> NAINPRLTPWTYRNTSFSSLPLTGENPGAWALVRDNSAKGITAGSGSQQTTYDPTRTEAALTASTTFALRRYDLAGRALYDLDFSKLNPQTPTRDQTGQITFNPFGGFGLSGAAPQQWNEVKNKVPVEVAQDPSNPYRFAVLLVPRSVVYYEQLQRGLGLPQQRTESGQNTSTTGAMFGLKVKNAEADTAKSNEKLQGAEATGSSTTSGSGQSTQRGGSSGDTKVKALKIEVKKKSDSEDNGQLQLEKNDLANAPIKRSEESGQSVQLKADDFGTALSSSGSGGNSNPGSPTPWRPWLATEQIHKDLPKWSASILILYDAPYARNRTAIDRVDHLDPKAMTANYPPSWRTPKWNHHGLWDWKARDVLLQTTGFFNPRRHPEWFDGGQTVADNEKTGFDVDNSENTKQGFQKEADSDKSAPIALPFEAYFANIGNLTWFGQALLVFGGNGHVTKSAHTAPLSIGVFRVRYNATGTSATVTGWPYALLFSGMVNKQTDGLKDLPFNNNRWFEYVPRMAVAGAKFVGRELVLAGTITMGDTATVPRLLYDELESNLNLVAQGQGLLREDLQLFTPYGWANRPDLPIGAWSSSSSSSHNAPYYFHNNPDWQDRPIQNVVDAFIKPWEDKNGKDDAKYIYPYRYSGMWAWQVYNWSNKLTDQPLSADFVNENAYQPNSLFAAILNPELLAALPDKVKYGKENEFAANEYERFNQKLTVAPTQGTNWSHFSPTLSRFSTGFNLVGSVLDQVLDYVPWIGNGYRYGNNHRGVDDITAPQTSAGSSSGISTNTSGSRSFLPTFSNIGVGLKANVQATLGGSQTMITGGSPRRTLDQANLQLWTGAGWRNDKASSGQSDENHTKFTSATGMDQQGQSGTSAGNPDSLKQDNISKSGDSLTTQDGNAIDQQEATNYTNLPPNLTPTADWPNALSFTNKNNAQRAQLFLRGLLGSIPVLVNRSGSDSNKFQATDQKWSYTDLHSDQTKLNLPAYGEVNGLLNPALVETYFGNTRAGGSGSNTTSSPGIGFKIPEQNNDSKATLITPGLAWTPQDVGNLVVSGTTVSFQLGGWLVTFTDFVKPRAGYLGLQLTGLDASDATQRALIWAPRPWAAFRGSWVNRLGRVESVWDLKGVWADQAQSDSQGSTTTATRNALPEHPNALAFQVSVVEASAYKPNTSSGQTQSTNSSPYLHLVKPKKVTQSDKLDDDLKNLLDPNQVRTKLRQSFGTDHSTQPQPQSLKTTTPVFGTSSGNLSSVLSGGGAGGGSSGSGQSGVDLSPVEKVSGWLVGQLPSTSDGNTSSTNNLAPNTNTGNDVVGVGRLSESNAAKMNDDVDGIVRT

M. pneumoniae binds to host target cells by means of a polar structure known as the attachment organelle, and glides in the direction of this differentiated structure at a speed of ~1 µm/s. P1, together with the P40/P90 polypeptides, forms a transmembrane complex called the “Nap”. In the present work, we report the structures of M. pneumoniae proteins P1 and P40/P90 and of complexes of P40/P90 bound to sialylated oligosaccharides. The structural results reveal that P1 (1627 residues) and P40/P90 (1218 residues) present a similar overall organization and topology in the extracellular regions.

The structure of the ectodomain from P1 was also studied by single-particle analysis using cryo-EM. A total of 68,014 selected particles yielded a 3D EM map at an overall resolution of ∼2.9 Å, according to the gold-standard Fourier shell correlation (FSC) 0.143 criterion (see “Methods”). The structure of P1 consists of a large N-terminal domain, with Asn60 as the first residue visible in the X-ray and the cryo-EM maps, and a smaller C-terminal domain (residues Gly1395–Asp1521). The cryo-EM and X-ray maps of P1 are well defined for most of the N-terminal domain with the residues clearly identifiable, in general, in both maps. However, from residue Pro1388 to the C-end, a region that includes the hinge between domains and the whole C-terminal domain, the density in the cryo-EM map becomes weak, indicating that there are hinge-like movements between domains. In the crown there are 13 disordered loops, spanning 117 residues, which could not be built. These disordered regions, essentially the same in the X-ray and cryo-EM structures, are spread over the N-terminal domain surface. In the crystal structure, the C-terminal domain is anchored by crystal contacts and the density is clear and crisp, while in the top part of the crown, with few crystal contacts, temperature factors are high and chain tracing was difficult. Together the cryo-EM and X-ray maps provide accurate structural information about the whole P1 ectodomain, proving the mobility of domains with respect to one another and confirming the characteristic presence of a large number of disordered loops. In the cryo-EM map of P1, the weak density of the C-terminal domain indicates flexibility with respect to the N-terminal domain proving that P1 can experience significant conformational changes consistent with the observations that antibodies that bind to the C-terminal domain can interfere with the attachment and gliding of mycoplasma cells.>MADKELKFLVVDDFSTMRRIVRNLLKELGFNNVEEA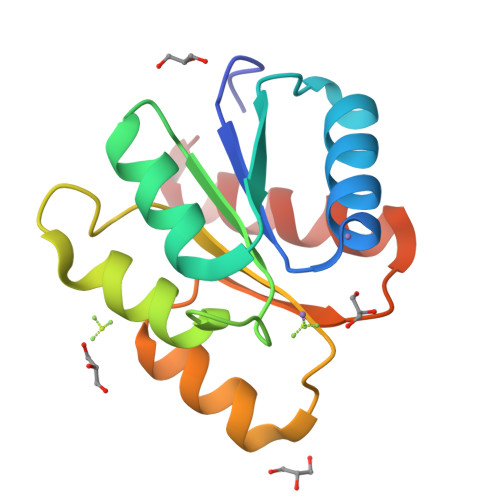EDGVDALNKLQAGGYGFVISDWNMPNMDGLELLKTIRADGAMSALPVLMVTSEAKKENIIAAAQAGASGYVVKPFTAATLEEKLNKIFEKLGM[2x]>CGGACCG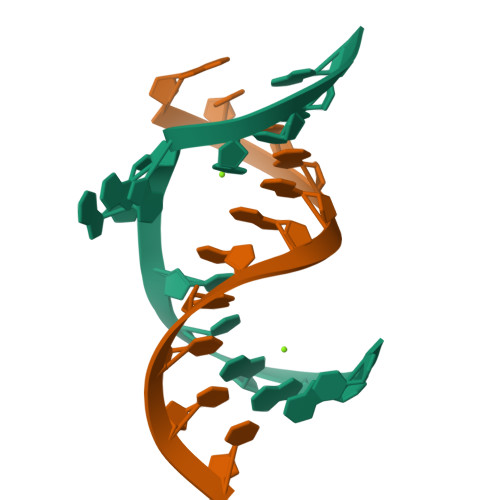AGCCAG[2x];>[2x]GCUGGGAGUCC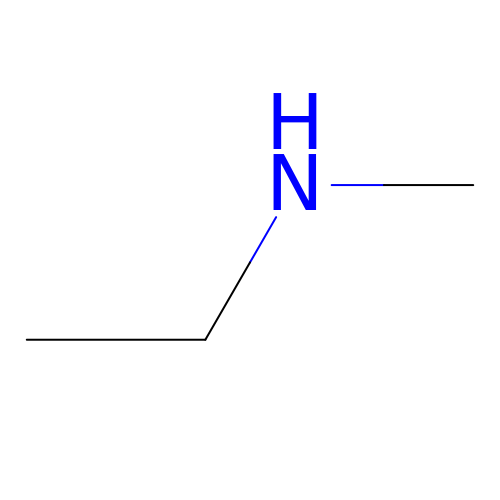METHYLETHYLAMINE | C3 H9 N | LIWAQLJGPBVORC-UHFFFAOYSA-N> KAQKKNRNKLRRQHSYDTF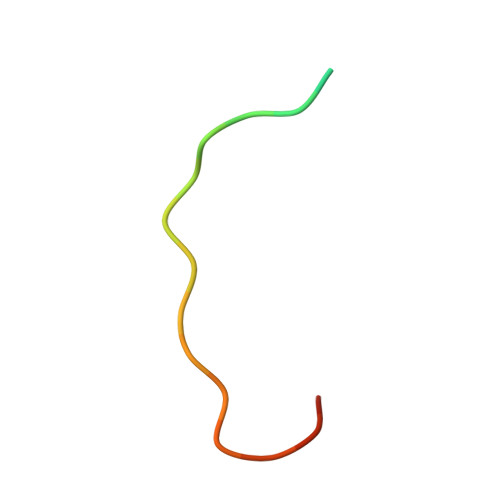VDL> MADSPNRLNRAKIDSTTMKDPRVLNNLKLRELLLPKFTSLWEIQTEVTVDNRTILLTWMHLLCESFELDKSVFPLSVSILDRYLCKKQGTKKTLQKIGAACVLIGSKIRTVKPMTVSKLTYLSCDCFTNLELINQEKDILEALKWDTEAVLATDFLIPLCNALKIPEDLWPQLYEA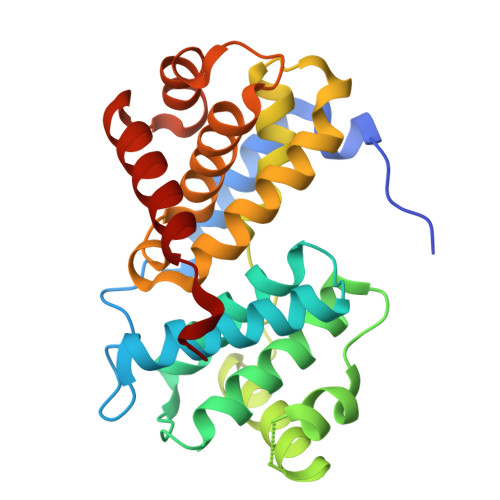ASTTICKALIQPNIALLSPGLICAGGLLTTIETDNTNCRPWTCYLEDLSSILNFSTNTVRTVKDQVSEAFSLYDLEIL>AEKPKLHYFNARGRMESTRWLLAAAGVEFEEKFIKSAEDLDKLRNDGYLMFQQVPMVEIDGMKLVQTRAILNYIASKYNLYGKDIKERALIDMYIEGIADLGEMILLLPVCPPEEKDAKLALIKEKIKNRYFPAFEKVLKSHGQDYLVGNKLSRADIHLVELLYYVEELDS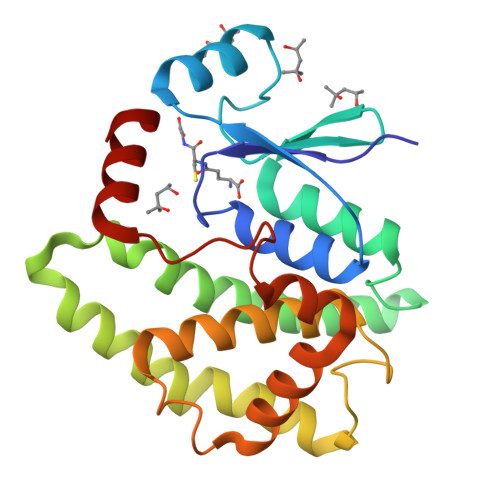SLISSFPLLKALKTRISNLPTVKKFLQPGSPRKPPMDEKSLEEARKIFRF[2x]>MNAPVFQQPHYEVVLDEGPDTINTSLITVQALDLDEGPNGTVTYAIVAGNIINTFRINKHTGVITAAKELDYEISHGRYTLIVTATDQCPILSHRLTSTTTVLVNVNDINDNVPTFPRDYEGPFDVTEGQPGPRVWTFLAHDRDSGPNGQVEYSVVDGDPLGEFVISPVEGVLRVRKDVELDRETIAF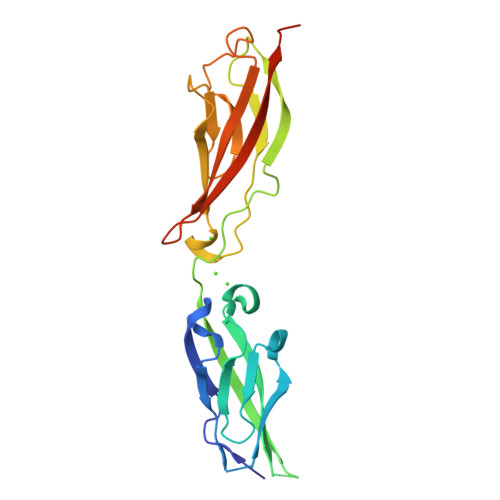YNLTICARDRGVPPLSSTMLVGIRVLDINDNLEHHHHHH[2x]> MATLNILVRNDKGRSSSYEVQLTQTVAVLKQQVCQRERVQADQFWLSFE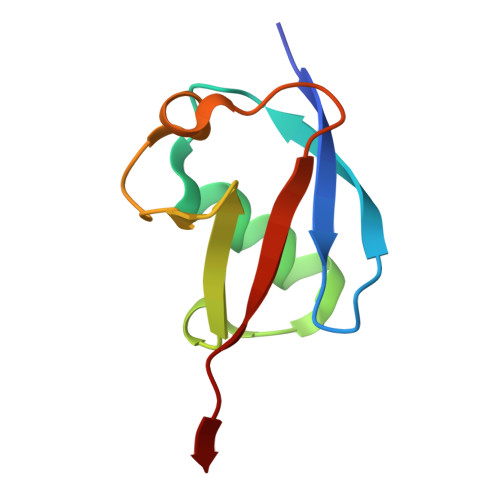GKPMDDEHPLGEYGLTTGCTVFMNLRLRG> MPFVNKQFNYKDPVNGVDIAYIKIPNAGQMQPVKAFKIHNKIWVIPERDTFTNPEEGDLNPPPEAKQVPVSYYDSTYLSTDNEKDNYLKGVTKLFERIYSTDLGRMLLTSIVRGIPFWGGSTIDTELKVIDTNCINVIQPDGSYRSEELNLVIIGPSADIIQFECKSFGHEVLNLTRNGYGSTQYIRFSPDFTFGFEESLEVDTNPLLGAGKFATDPAVTLAHELIHAGHRLYGIAINPNRVFKVNTNAYYEMSGLEVSFEELRTFGGHDAKFIDSLQENEFRLYYYNKFKDIASTLNKAKSIVGT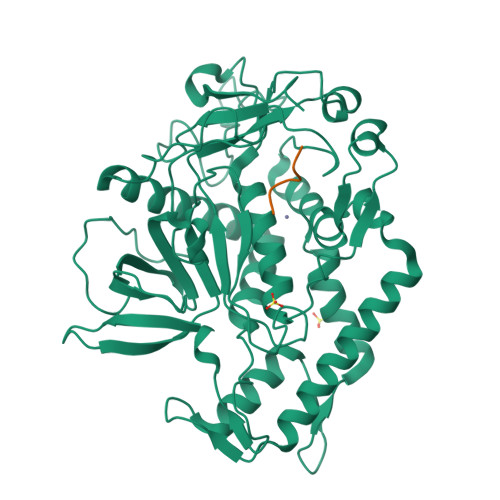TASLQYMKNVFKEKYLLSEDTSGKFSVDKLKFDKLYKMLTEIYTEDNFVKFFKVLNRKTYLNFDKAVFKINIVPKVNYTIYDGFNLRNTNLAANFNGQNTEINNMNFTKLKNFTGLFEHHHHHH;> RRATKMX> GAMDMYAPHSIRIEGDVTLGGLFPVHAKGPSGVPCGDIKRENGIHRLEAMLYALDQINSDPNLLPNVTLGARILDTCSRDTYALEQSLTFVQALIQKDTSDVRCTNGEPPVFVKPEKVVGVIGASGSSVSIMVANILRLFQIPQISYASTAPELSDDRRYDFFSRVVPPDSFQAQAMVDIVKALGWNYVSTLASEGSYGE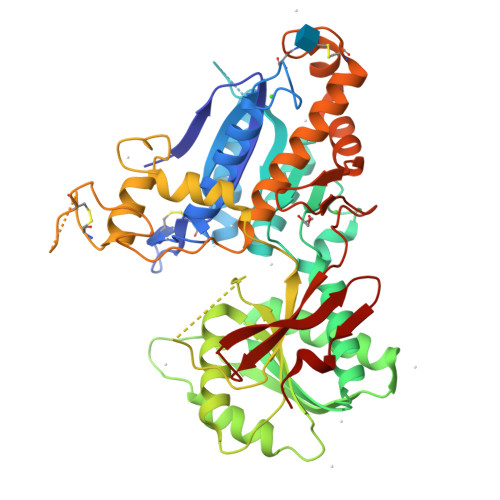KGVESFTQISKEAGGLSIAQSVRIPQERKDRTIDFDRIIKQLLDTPNSRAVVIFANDEDIKQILAAAKRADQVGHFLWVGSDSWGSKINPLHQHEDIAEGAITIQPKRATVEGFDAYFTSRTLENNRRNVWFAEYWEENFNCKLTISGSKKEDTDRKCTGQERIGKDSNYEQEGKVQFVIDAVYAMAHALHHMNKDLCADYRGVCPEMEQAGGKKLLKYIRNVNFNGSAGTPVMFNKNGDAPGRYDIFQYQTTNTSNPGYRLIGQWTDELQLNIEDMQWGK> GGGRGSGKEVRVPATALCVFDAHDGEVNAVQFSPGSRLLATGGMDRRVKLWEVFGAACEFKGSLSGSNAGITSIEFDSAGSYLLAASNDFASRIWTVDDYRLRHTLTGHSGKVLSAKFLLDNARIVSGSHDRTLK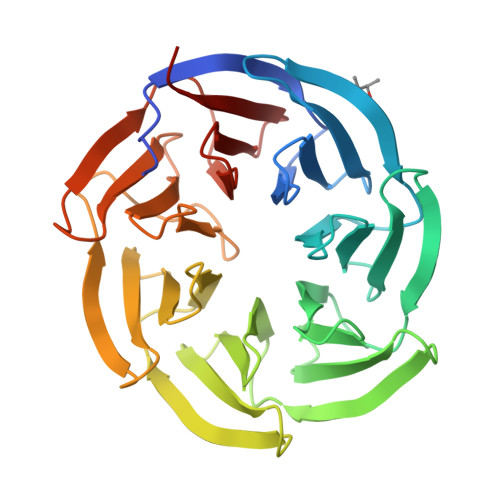LWDLRSKVCIKTVFAGSSCNDIVCTEQCVMSGHFDKKIRFWDIRSESIVREMELLGKITALDLNPERTELLSCSRDDLLKVIDLRTNAIKQTFSAPGFKCGSDWTRVVFSPDGSYVAAGSAEGSLYIWSVLTGKVEKVLSKQHSSSINAVAWSPSGSHVVSVDKGCKAVLWAQP> GAQVSSQKVGAHENSNRAYGGSTINYTTINYYRDSASNAASKQDFSQDPSKFTEPIKDVLIKTAPMLNSPNIEACGYSDRVLQLTLGNSTITTQEAANSVVAYGRWPEYLRDSEANPVDQPTEPDVAACRFYTLDTVSWTKESRGWWWKLPDALRDMGLFGQNMYYHYLGRSGYTVHVQCNA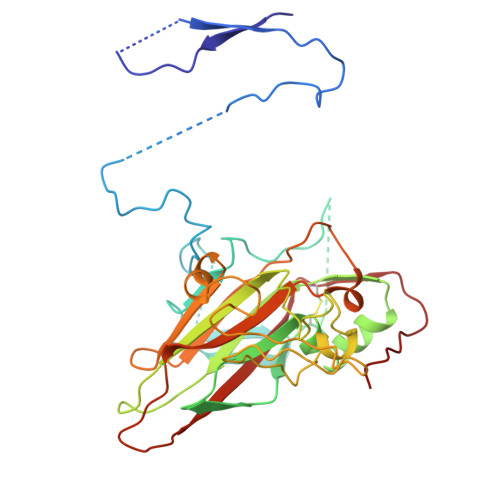SKFHQGALGVFAVPEMCLAGDSNTTTMHTSYQNANPGEKGGTFTGTFTPDNNQTSPARRFCPVDYLLGNGTLLGNAFVFPHQIINLRTNNCATLVLPYVNSLSIDSMVKHNNWGIAILPLAPLNFASESSPEIPITLTIAPMCCEFNGLRNITLPRLQ>ADSDINIKTGTTDIGSNTTVKTGDLVTYDKENGMHKKVFYSFIDDKNHNKKLLVIRTKGTIAGQYRVYSEEGANKSGLAWPSAFKVQLQLPDNEVAQISDYYPRNSIDTKEYMSTLTYGFNGNVTGDDTGKIGGLIGANVSIG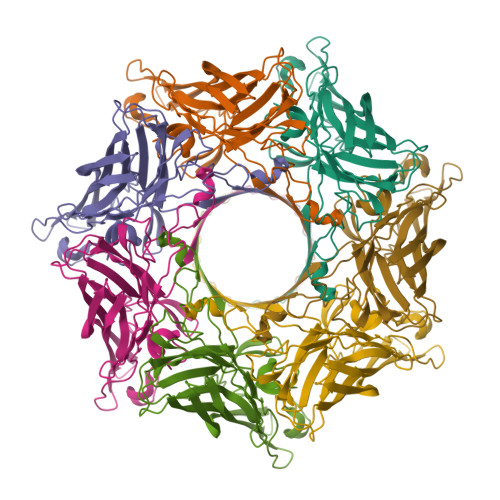HTLKYVQPDFKTILESPTDKKVGWKVIFNNMVNQNWGPYDRDSWNPVYGNQLFMKTRNGSMKAADNFLDPNKASSLLSSGFSPDFATVITMDRKASKQQTNIDVIYERVRDDYQLHWTSTNWKGTNTKDKWTDRSSERYKIDWEKEEMTN[7x]Cyclodipeptide synthases (CDPSs) use aminoacylated tRNA (aa-tRNA) substrates to form peptide bonds between two amino acids yielding a cyclic dipeptide product (CDP). ParaCDPS from Parabacteroides sp. 20_3 (GenBank: EFK64745.1) produces cyclo(His-Phe)8 whilst ParcuCDPS from Parcubacteria bacterium RAAC4_OD1_1 (GenBank: ETB63777.1) can synthesise both cyclo(His-Glu) and cyclo(His-Pro)9. ParcuCDPS belongs to the XYP sub-group of the CDPS family, characterised by the presence of 3 residues: X40 where X is a non-conserved residue, Y202, and P203 (numbering respective to AlbC). ParcuCDPS displays a Rossman-fold common throughout the CDPS family.

Additionally, we hypothesised D58 was acting as a potential active site residue, within hydrogen bond distance from the catalytic serine (S26), which could be important for S26 to act as a nucleophile. In the common CDPS fold helix α3 and α4 exist as a single continuous helix whereas, in ParcuCDPS a flexible glycine residue (G84) provides a significant bend and change of direction, splitting the helix into two. β3 holds another important deviation seen in ParcuCDPS’ structure, as it changes direction (compared to common CDPS fold) at I56 to divide the active site pocket. This structural change of β3 facilitates the placement of D58 into H-bonding distance of the active site S26. The active site mutants – S26A; S26C; D58A; D58N; Y167A; Y167F; E171A; and E171Q—were also generated to confirm the loss of activity upon removing catalytic residues. Indeed, when the hydrogen bond between S26 and D58 is disrupted by mutating D58 to either an alanine or an asparagine, ParcuCDPS loses over 90% of activity, while preserving its structure. When the H-bond between S26 and D58 is disrupted by mutating D58 to either an alanine or an asparagine, the enzyme is inactive (activity < 1% WT). This highlights the essential role that D58 has in potentially polarizing and positioning the serine in the active site for substrate binding and acyl enzyme formation. Further investigation into the changes imposed by these mutants was performed by solving the crystal structures of a select few mutants containing changes to the active site or the pocket residues. The mutant structures were able to be solved using WT as a model and retained an equivalent fold to ParcuCDPS (Supplementary Notes 4 and 7 relating to Supplementary Figs. 13 and 14). Therefore, the disruption of activity is caused exclusively by the change in these few residues which appear important for the enzyme to produce a CDP.

> MELHQIRGCHKNDIELKKYNIGVAISLGNKWFSIDNIEKLVKWSLLHTKEYVIIYIANSIHGINLSVRNKLSDSHAEEVAIRYGRNLFIKIKERVSLSFSQDEQAKIIYATWSDIADSKYKEKVKYLYNLYDKNINFKNYIENFVKEWVSKEKRTFNNNEINKFGRYILEELPELMVQVKARGVLFEAYVYPYKTRITEFVGLLQKGEIFPEIKTNILDNHPKIFLEVREHHHHHH>MIPVTELRYFADTQPAYRILKPWWDVFTDYISIVMLMIAVFGGTLQVTQDKMICLPCKWVTKDSCNDSFRGWAAPGPEPTYPNSTILPTPDTGPTGIKYDLDRHQYNYVDAVCYENRLHWFAKYFPYLVLLHTLIFLACSNFWFKFPRTSSKLEHFVSILLKCFDSPWTTRALSETVVEESDPKPAFSKMNGSMDKKSSTVSEDVEATVPMLQRTKSRIEQGIVDRSETGVLDKKEGEQAKALFEKVKKFRTHVEEGDIVYRLYMRQTIIKVIKFILIICYTVYYVHNIKFDVDCTVDIESLTGYRTYRCAHPLATLFKILASFYISLVIFYGLICMYTLWWMLRRSLKKYSFESIREESSYSDIPDVKNDFAFMLHLIDQYDPLYSKRFAVFLSEVSENKLRQLNLNNEWTLDKLRQRLTKNAQDKLELHLFMLSGIPDTVFDLVELEVLKLELIPDVTIPPSIAQLTGLKELWLYHTAAKIEAPALAFLRENLRALHIKFTDIKEIPLWIYSLKTLEELHLTGNLSAENNRYIVIDGLRELKRLKVLRLKSNLSKLPQVVTDVGVHLQKLSINNEGTKLIVLNSLKKMANLTELELIRCDLERIPHSIFSLHNLQEIDLKDNNLKTIEEIISFQHLHRLTCLKLWYNHIAYIPIQIGNLTNLERLYLNRNKIEKIPTQLFYCRKLRYLDLSHNNLTFLPADIGLLQNLQNLAITANRIETLPPELFQCRKLRALHLGNNVLQSLPSRVGELTNLTQIELRGNRLECLPVELGECPLLKRSGLVVEEDLFNTLPPEVKERLWRADKEQATGGLVPR[6x];>MAMPEKRPFERLPADVSPINYSLCLKPDLLDFTFEGKLEAAAQVRQATNQIVMNCADIDIITASYAPEGDEEIHATGFNYQNEDEKVTLSFPSTLQTGTGTLKIDFVGELNDKMKGFYRSKYTTPSGEVRYAAVTQFEATDARRAFPCWDEPAIKATFDISLVVPKDRVALSNMNVIDRKPYPDDENLVEVKFARTPVMSTYLVAFVVGEYDFVETRSKDGVCVRVYTPVGKAEQGKFALEVAAKTLPFYKDYFNVPYPLPKIDLIAIADFAAGAMENWGLVTYRETALLIDPKNSCSSSRQWVALVVGHELAHQWFGNLVTMEWWTHLWLNEGFASWIEYLCVDHCFPEYDIWTQFVSADYTRAQELDALDNSHPIEVSVGHPSEVDEIFDAISYSKGASVIRMLHDYIGDKDFKKGMNMYLTKFQQKNAATEDLWESLENASGKPIAAVMNTWTKQMGFPLIYVEAEQVEDDRLLRLSQKKFCAGGAYVGEDCPQWMVPITISTSEDPNQAKLKILMDKPEMNVVLKNVKPDQWVKLNLGTVGFYRTQYSSAMLESLLPGIRDLSLPPVDRLGLQNDLFSLARAGIISTVEVLKVMEAFVNEPNYTVWSDLSCNLGILSTLLSHTDFYEEIQEFVKDVFSPIGERLGWDPKPGEGHLDALLRGLVLGKLGKAG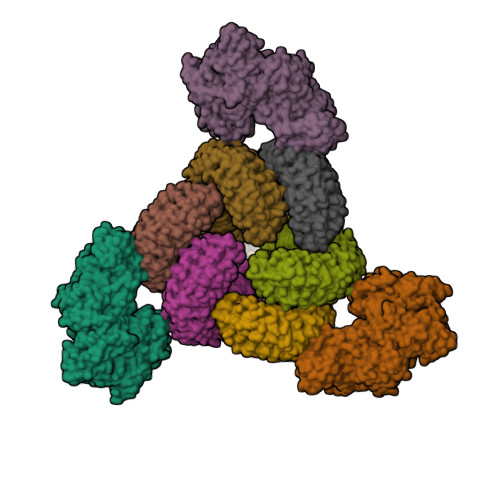HKATLEEARRRFKDHVEGKQILSADLRSPVYLTVLKHGDGTTLDIMLKLHKQADMQEEKNRIERVLGATLLPDLIQKVLTFALSEEVRPQDTVSVIGGVAGGSKHGRKAAWKFIKDNWEELYNRYQGGFLISRLIKLSVEGFAVDKMAGEVKAFFESHPAPSAERTIQQCCENILLNAAWLKRDAESIHQYLLQRKASPPTVTGGLVPR[3x]> GHMSFVITNPEALTVAATEVRRIRDRAIQSDAQVAPMTTAVRPPAADLVSEKAATFLVEYARKYRQTIAAAAVVLEEFAHALTTGADKYATAEADNIKTFS;> MHFEAYPPEVNSANIYAGPGPDSMLAAARAWRSLDVEMTAVQRSFNRTLLSLMDAWAGPVVMQLMEAAKPFVRWLTDLCVQLSEVERQIHEIVRAYEWAHHDMVPLAQIYNNRAERQILIDNNLLGQFTAQIADLDQEYDDFWDEDGEVMRDYRLRVSDALSKLTPWKAPPPIAHS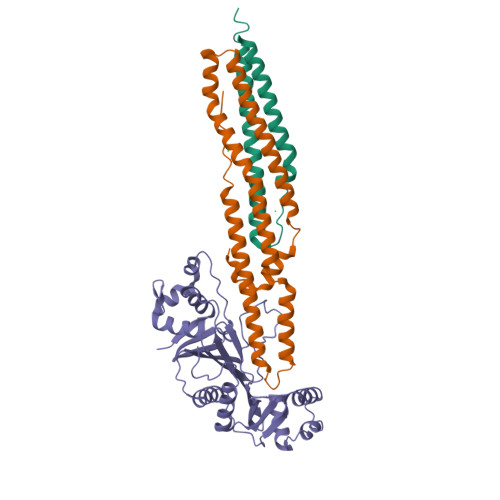TVLVAPVSPSTASSRTDT;> MDQQSTRTDITVNVDGFWMLQALLDIRHVAPELRCRPYVSTDSNDWLNEHPGMAVMREQGIVVGDTVNEQVAARMRVLAAPDLEVVALLSRGKLLYGVVDNEDQPPGSRDIPDNEFRVVLARRGQHWVSAVRVGNDITVDDVSVSDSASIAALVIDGLESIHHADPAAINAVNVPLEEMLEATKSWQESGFNVFSGGDLRRMGISASTVAALGQALSDPAAEVAVYARQYRDDAKGPSASVLSLKDGSGGRIALYQQARTAGSGEAWLAICPATPQLVQVGVKTVLDTLPYGEWKTHSRV> MNSPVDAPKWPRQIPYIIASEACERFSFYGMRNILTPFLMTALLLSIPEELRGAVAKDVFHSFVIGVYFFPLLGGWIADRFFGKYNTILWLSLIYCVGHAFLAIFEHSVQGFYTGLFLIALGSGGIKPLVSSFMGDQFDQSNKSLAQKAFDMFYFTINFGSFFASLSMPLLLKNFGAAVAFGIPGVLMFVATVFFWLGRKRYIHMPPEPKDPHGFLPVIRSALLTKVEGKGNIGLVLALIGGVSAAYALVNIPTLGIVAGLCCAMVLVMGFVGAGASLQLERARKSHPDAAVDGVRSVLRILVLFALVTPFWSLFDQKASTWILQANDMVKPQWFEPAMMQALNPLLVMLLIPFNNFVLYPAIERMGVKLTALRKMGAGIAITGLSWIVVGTIQLMMDGGSALSIFWQILPYALLTFGEVLVSATGLEFAYSQAPKAMKGTIMSFWTLSVTVGNLWVLLANVSVKSPTVTEQIVQTGMSVTAFQMFFFAGFAILAAIVFALYARSYQMQDHYRQATGSENLYFQ

Proton-coupled oligopeptide transporters belong to the major facilitator superfamily (MFS) of membrane transporters. PepT1 is a member of the POT family of proton-dependent oligopeptide transporters (TC 2.A.17), which itself belongs to the much larger major facilitator superfamily (MFS) of secondary active transport proteins (Reddy et al., 2012). Peptide transporters are proton-coupled symporters and use the inwardly directed proton electrochemical gradient to drive peptide uptake into the cell. Using modeling, molecular dynamics, crystallography, functional assays, and site-directed spin labeling combined with double electron-electron resonance (DEER) spectroscopy, we present a detailed study of the transport dynamics of two bacterial oligopeptide transporters, PepTSo and PepTSt.

The existing inward-occluded structure of PepTSo (Newstead et al., 2011) was found to be not suitable for constructing a repeat-swapped model due to asymmetries between the N- and C-terminal halves of the protein, which led to steric hindrance problems during model building. First, a lateral helix between H6 and HA is resolved for the first time. Second, the residues that make up the cytoplasmic thin gate adopt different positions, such that this structure is inward open (the new PepTSo structure thus resembles the previously reported inward-open PepTSt structure). Third, some weak difference density (Fo − Fc) is present in a position equivalent to that observed in the previous structure, indicating that this crystal structure may not represent a fully inward-open, ligand-free state. Fourth, a solvent-accessible cavity is observed in the new structure that permits protons to access the ExxERF motif on H1. This motif has previously been shown to play an important role in proton-coupled transport (Solcan et al., 2012). The resulting pore profiles confirm that the central cavity in the new structure of PepTSo is accessible to the cytoplasm but inaccessible to the periplasm, hence the structure can be described as inward open. The repeat-swapping method was applied to both this structure of PepTSo and the existing inward-open structure of PepTSt, generating outward-facing models of both proteins. Although these two residues are not interacting with one another in the inward-facing structure of PepTSo, again only comparatively small motions would be required to bring this about. Examining the structure of PepTSo suggests that the kink in H8 is due to two prolines, P345 and P353 (P329 and P345 in PepTSt), the latter being highly conserved across the POT family.>GPGSAEKKVEAKVEVAENNVSSVARREKELYDQIADLTDKNGEYLERIGELEERQKNLEKLEHQSQVAADKHYQEQAKKHQEYKQEQEER[2x];>GPGSNCGPPPTLSFAAPMDITLTETRFKTGTTMKYTCLPGYVRSHSTQTMTCNSDGEWVYNTFCIYKRCRHPGELRNGQVEIKTDLSFGSQIEFSCSEGFFLIGSTTSRCEVQDRGVGWS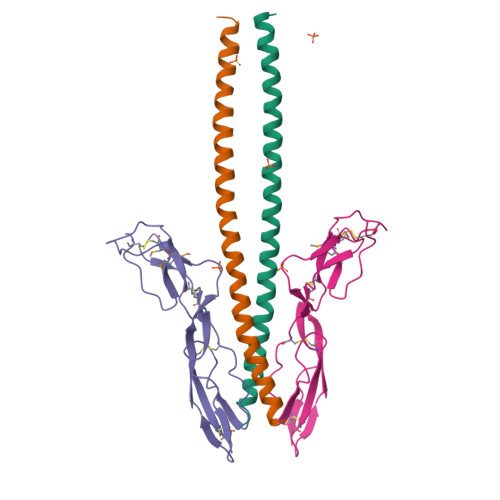HPLPQCEI[2x]> LRSANPTIAKALQPLIEGPKFAVVYCGNHQYKV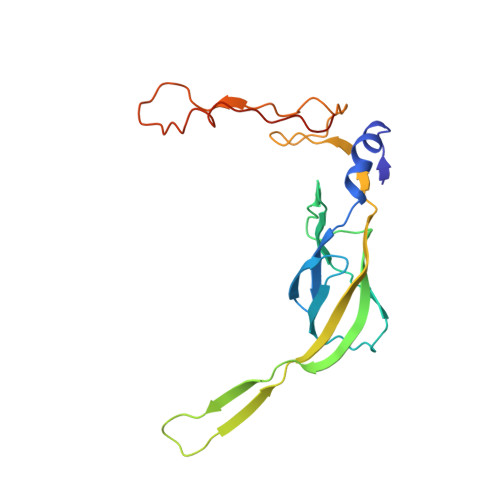SPGDVIAVQRLRAPIGSQIALKKVLMVGGPRFTAIGRPLLEHVRVTADVEEQKRMRNVVSLFSTPGRRRLRWLDAQHAATILRIREVVYEPTVVGELDKYDGVLLKDFHADRHPNPVFTANDGYDLYYPKDWNKVEEASAFLEMMEAPPTEK> GSHMAALRERAGPVTWVMMIACVVVFI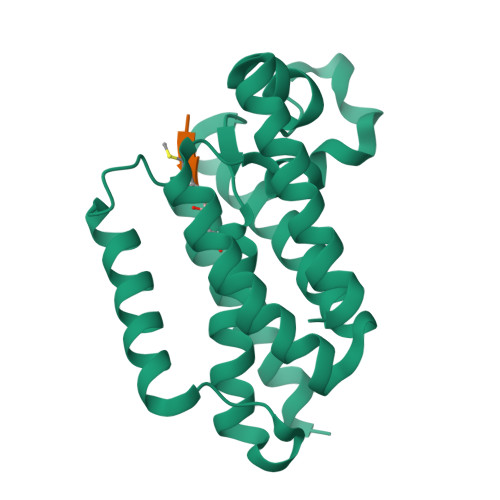AMQILGDQEVMLWLAWPFDPTLKFEFWRYFTHALMHFSLMHILFNLLWWWYLGGAVEKRLGSGKLIVITLISALLSGYVQQKFSGPWFGGLSGVVYALMGYVWLRGERDPQSGIYLQRGLIIFALIWIVAGWFDLFGMSMANGAHIAGLAVGLAMAFVDSLNARKRK;> XVRMA>[2x]SAARRAGTSCANCQTTTTTLWRRNANGDPVCNACGLYYKLHNINRPLTMKKEGIQT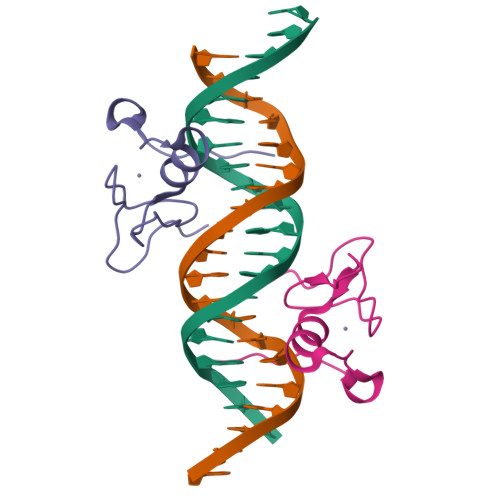RNRKMSS>[2x]TGTPVERYGKVQVCGTQLCDEHGNP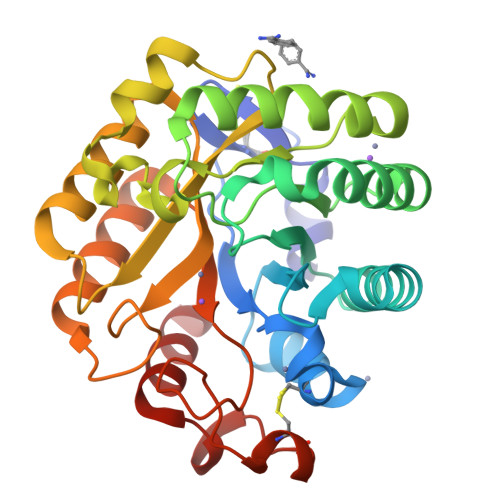VQLRGMSTHGIQWFDHCLTDSSLDALAYDWKADIIRLSMYIQEDGYETNPRGFTDRMHQLIDMATARGLYVIVDWHILTPGDPHYNLDRAKTFFAEIAQRHASKTNVLYEIANEPNGVSWASIKSYAEEVIPVIRQRDPDSVIIVGTRGWSSLGVSEGSGPAEIAANPVNASNIMYAFHFYAASHRDNYLNALREASELFPVFVTEFGTETYTGDGANDFQMADRYIDLMAERKIGWTKWNYSDDFRSGAVFQPGTCASGGPWSGSSLKASGQWVRSKLQS> MGHHHHHHMLHLLEQIRAYCETCWEWQEAHEPGMDQDKNPMPAPVEHQICPAVCVLMKLSFDEEHRHAMNELGGLQAIAELLQVDCEMYGLTNDHYSITLRRYAGMALTNLTFGDVANKATLCSMKGCMRALVAQLKSESEDLQQVIASVLRNLSWRADVNSKK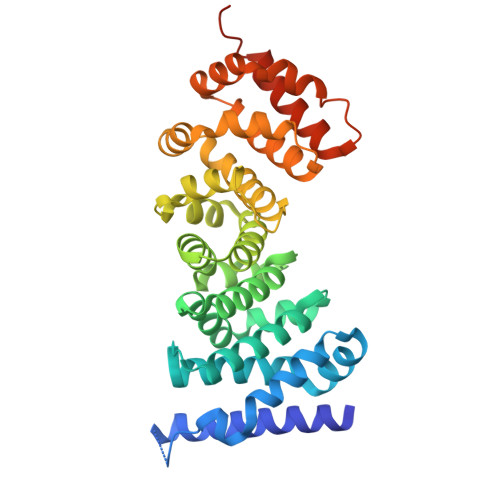TLREVGSVKALMECALEVKKESTLKSVLSALWNLSAHCTENKADICAVDGALAFLVGTLTYRSQTNTLAIIESGGGILRNVSSLIATNEDHRQILRENNCLQTLLQHLKSHSLTIVSNACGTLWNLSARNPKDQEALWDMGAVSMLKNLIHSKHKMIAMGSAAALRNLMANRPAKYKDANIMSPGSSLPS> MWSHPQFEKASSDNSANKRIQSGGCAIHCQDCSISQLCIPFTLNDSELDQLDEIIERKKPIQKGQELFKAGDELKCLYAIRSGTIKSYTITEQGDEQITAFHLAGDLVGFDAITEAQHPSFAQALET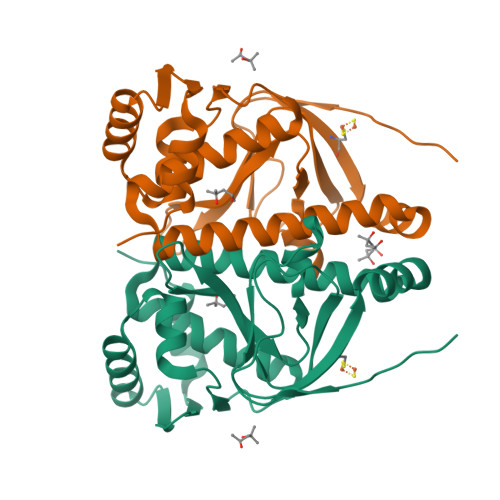SMVCEIPYEILDDLSGKMPKLRQQIMRLMSNEIKGDQEMILLLSKKNAEERLAAFLYNLSTRFHQRGFSPREFRLTMTRGDIGNYLGLTVETISRLLGRFQKTEMLTVKGKYITINDHDALAELAGSAKEIK> MAATAAEAVTSGSGEPREEAGALGPAWDESQLRSYSFPTRPIPRLSQSDPRAEELIENEEPVVLTDTNLVYPALKWDLEYLQENIGNGDFSVYSASTHKFLYYDEKKMANFQNFKPRSNREEMKFHEFVEKLQDIQQRGGEERLYLQQTLNDTVGGKIVMDFLGFNWNWINKQQGKRGWGQLTSNLLLIGMEGNVTPAHYDEQQNFFAQIKGYKRCILFPPDQFECLYPYPVHHPCDRQSQVDFDNPDYERFPNFQNVVGYETVVGPGDVLYIPMYWWHHIESLLNGGITITVNFWYKGAPTPKRIEYPLKAHQKVAIMRNIEKMLGEALGNPQE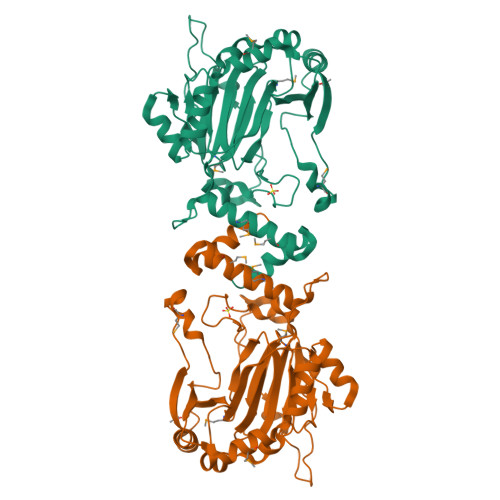VGPLLNTMIKGRYN>AVTGQVDVKLNISTGCTVGGSQTEGNMNKFGTLNFGKTSGTWNNVLTAEVASAATGGNISVTCDGTDPVDFTVAIDGGERTDRTLKNTASADVVAYNVYRDAARTNLYVVNQPQQFTTVSGQATAVPIFGAIAPNTGTPKAQGDYKDTLL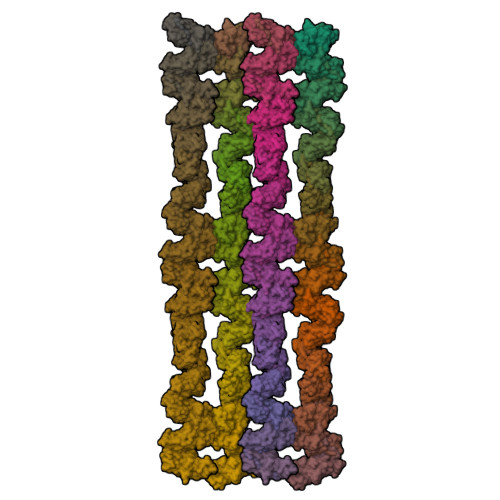VTVNF[72x]deoxysordaricin | C20 H28 O3 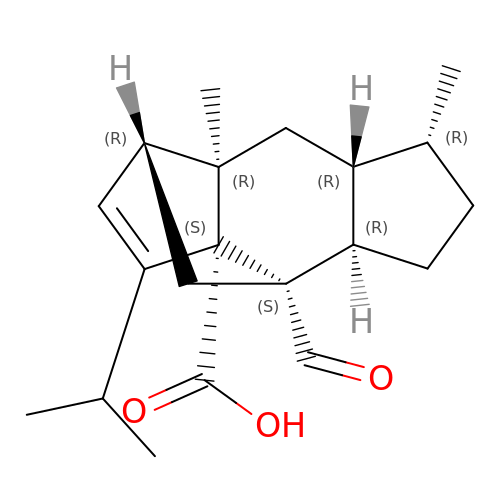| PREPDMQKKFKALX-JUZOJGAKSA-N NHLRC2 (NHL repeat containing protein 2) is an essential cytosolic protein of unknown function, mutation of which was recently identified in association with FINCA (fibrosis, neurodegeneration, cerebral angiomatosis) disease, a multi-organ condition which is fatal in early childhood. NHLRC2 contains three domains; an N-terminal thioredoxin-like (Trx-like) domain, followed by a six-bladed NHL repeat containing β-propeller domain and then a C-terminal β-stranded domain. The N-terminal Trx-like domain contains a CCINC motif at the position of the CXXC motif, which is characteristic of oxidoreductases and commonly involved in thiol-disulfide exchange. The six-bladed β-propeller domain comprises six NHL repeats, a structural motif originally identified in genes NCL-1, HT2A and LIN-41 and shown to often function as a protein-protein interaction module.

The crystal structure of the β-propeller domain was solved by single-wavelength anomalous dispersion method using selenomethionine substituted protein. The crystals of native β-propeller domain diffracted to 1.75 Å, belong to a space group P21 and contain one molecule of the β-propeller in the asymmetric unit. Given the high resolution of the data, the electron density for the main-chain is complete and side chain residues are clearly visible, except for a short fragment between residues 346 and 352 where the electron density is missing. The β-propeller domain of NHLRC2 comprises six blades containing four twisted antiparallel β-strands, labeled A–D from the inside to the outside of the molecule, arrayed around a central pseudo-sixfold axis. In contrast to other β-propeller proteins, the NHLRC2 β-propeller is not closed by a so called ‘Velcro strap’ which is the insertion of the first N-terminal β-strand into the last propeller blade framework. Instead, N- and C-terminal β-strands even though located in close proximity to each other, belong to separate β-propeller blades. The central pore of the β-propeller domain of NHLRC2 is approximately 12 Å in diameter and contains a number of water molecules. The continuous water channel is disrupted by hydrogen bonds which Lys-228 and Asp-340 form with water and backbone groups of adjacent blades. No electron density corresponding to metal ions were observed in the NHLRC2 β-propeller structure and structure-based alignment does not reveal any relevant residues which might participate in a catalytic reaction. Together this suggests that the domain does not function as an enzyme, but rather that the NHLRC2 β-propeller domain is involved in protein-protein interaction(s).

> MHHHHHHMSPLLFPGKVTVDQVTDRLVIADTGHHRILVVWKNGQIQYSIGGPNPGRKDGIFSESTFNSPQGVAIMNNIIYVADTENHLIRKIDLEAEKVSTVAGIGIQGTDKEGGAKGEQQPISSPWDVVFGTSGSEVQRGDILWIAMAGTHQIWALLLDSGKLPKKNELTKGTCLRFAGSGNEENRNNAYPHKAGFAQPSGLSLASEDPWSCLFVADSESSTVRTVSLKDGAVKHLVGGERDPMNLFAFGDVDGVGINAKLQHPLGVTWDKKRNLLYVADSYNHKIKVVDPKTKNCTTLAGTGDTNNVTSSSFTESTFNEPGGLCIGENGELLYVADTNNHQIKVMDLETKMVSVLPIF> MNDQPFAWQVASLSERYQEQFDIGAAVEPYQLEGRQAQILKHHYNSLVAENAMKPESLQPREGEWNWEGADKIVEFARKHNMELRFHTLVWHSQVPEWFFIDEDGNRMVDETDPDKREANKQLLLERMENHIKTVVERYKDDVTSWDVVNEVIDDGGGLRESEWYQITGTDYIKVAFETARKYGGEEAKLYINDYNTEVPSKRDDLYNLVKDLLEQGVPIDGVGHQSHIQIGWPSIEDTRASFEKFTSLGLDNQVTELDMSLYGWPPTGAYTSYDDIPAELLQAQADRYDQLFELYEELAADI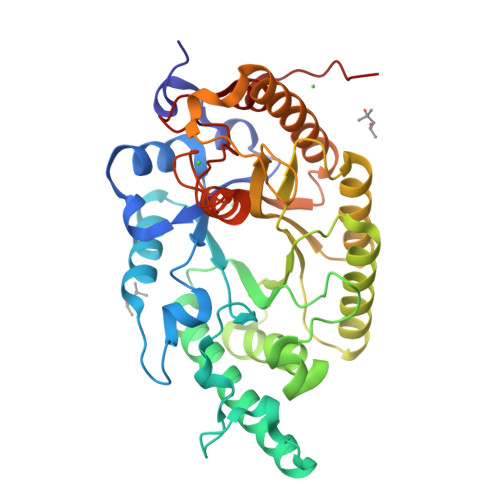SSVTFWGIADNHTWLDGRAREYNNGVGIDAPFVFDHNYRVKPAYWRIIDLEHHHHHH>GSGMLGMYVPD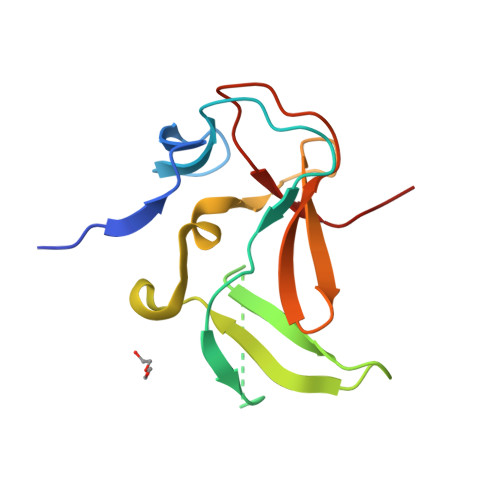RFSLKSSRVQDGMGLYTARRVRKGEKFGPFAGEKRMPEDLDENMDYRLMWEVRGSKGEVLYILDATNPRHSNWLRFVHEAPSQEQKNLAAIQEGENIFYLAVEDIETDTELLIGYLDSD[2x]>[3x]MSEMTPREIVSELDQHIIGQADAKRAVAIALRNRWRRMQLQEPLRHEVTPKNILMIGPTGVGKTEIARRLAKLANAPFIKVEATKFTEVGYVGKEVDSIIRDLTDSAGGAIDAVEQNGIVFIDEIDKICKKGEYSGADVSREGVQRDLLPLVEGSTVSTKHGMVKTDHILFIASGAFQVARPSDLIPELQGRLPIRVELTALSAADFERILTEPHASLTEQYK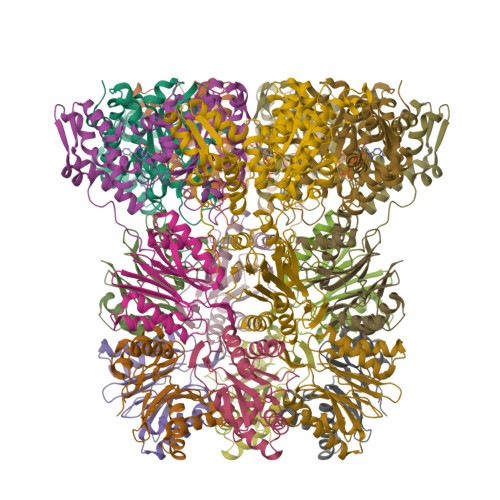ALMATEGVNIAFTTDAVKKIAEAAFRVNEKTENIGARRLHTVMERLMDKISFSASDMNGQTVNIDAAYVADALGEVVENEDLSRFIL;>[6x]TTIVSVRRNGQVVVGGDGQVSLGNTVMKGNARKVRRLYNGKVLAGFAGGTADAFTLFELFERKLEMHQGHLLKSAVELAKDWRTDRALRKLEAMLIVADEKESLIITGIGDVVQPEEDQILAIGSGGNYALSAARALVENTELSAHEIVEKSLRIAGDICVFTNTNFTIEELPN>[2x]DEFQWKGLPVVKSGLDVGGMPTGTRYHRSPAWPEEQPGETHAPAPFGSGDKRYTFSQTEMLVNGLKPYTEPTAGVPPQLLSRAVTHVRSYIETIIGTHRSPVLTYHQACELLERTTSCGPFVQGLKGDYWDEEQQQYTGVLANHLEQAWDKANKGIAPRNAYKLALKDELRPIEKNKAGKRRLLWGCDAATTLIATAAFKAVATRLQVVTPMTPVAVGINMDSVQMQVMNDSLKGGVLYCLDYSKWDSTQNPAVTAASLAILERFAEPHPIVSCAIEALSSPAEGYVNDIKFVTRGGLPSGMPFTSVVNSINHMIYVAAAILQAYESHNVPYTGNVFQVETIHTYGGGCMYSVCPATASIFHTVLANLTSYGLKPTAADKSDAIKPTNTPVFLKRTFTQTPHGIRALLDITSITRQFYWLKANRTSDPSSP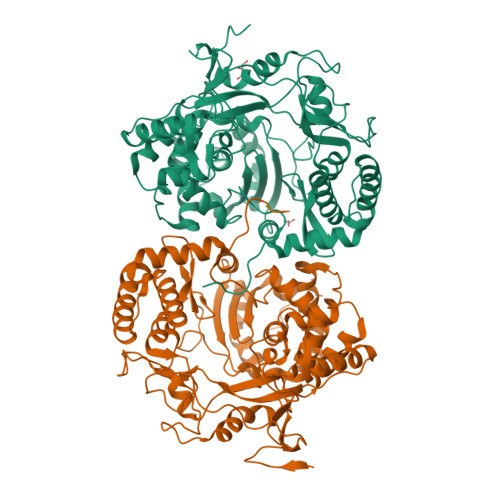PAFDRQARSAQLENALAYASQHGPVMFDTVRQIAIKTAQGEGLVLVNTNYDQALATYNAWFIGGTVPDPVGHTEGTHKIVFEME>MAGAIKVGTWGGNGGSEWDMGPAYRIDSVKINAGDIIDAIEITFTRYGLTETQHYGGTGGEPHEIAFEDGEYIMSMEGHVVDYTGLTIIGKLTLTTNRRTFGPFGAYEGTPFSIPVAEGKIAGFFGRAGSFIDAIGVYLMPNLEHHHHHH[16x]

A BLAST protein sequence alignment search revealed a candidate lectin from Musa acuminata ssp. malaccensis, which we term Malayasian banana lectin (Malay BanLec). Like BanLec, Malay BanLec has a β-prism-I fold characteristic of the jacalin-related lectin family. To assess binding of WT versus F84T to HIV, we conducted surface plasmon resonance analysis to determine the binding times to, and binding avidities for, the gp140 trimer, which is made up of uncleaved ectodomains of the gp160 HIV envelope glycoprotein trimer. The results show that F84T and WT Malay BanLec, which like BanLec exist as dimers with two CBS per monomer (see Fig. 6 below and discussion thereof), bind with high avidity to the gp140 trimer. That is, we asked whether disruption of pi–pi stacking in a structurally related but distinct (only 63% identical at the amino acid level) jacalin-related lectin, Malaysian banana lectin (Malay BanLec), would reduce mitogenicity of the engineered lectin without abolishing antiviral activity.

We demonstrate that a single amino acid substitution, F84T, akin to the H84T mutation and predicted to remove the pi–pi stacking interaction, does indeed decrease mitogenicity while preserving antiviral activity. The F84T mutation in Malay BanLec disrupts pi–pi stacking without significant changes to the overall structure of the monomer or to the dimer. F84T and WT Malay BanLec have an almost identical structure, with an RMSD of 0.424 Å between all atoms. F84T Malay BanLec similarly loses pi–pi stacking (the “mitogenic wall”), but otherwise retains a structure that is almost identical to its parent lectin. We thus conclude that F84T is less mitogenic than is WT Malay BanLec because it likely does not crosslink surface molecules as well. F84T-treated cells also incorporated less BrdU than WT Malay BanLec-treated cells, indicating that F84T is less mitogenic than WT Malay BanLec. Taken together, these studies indicate that F84T induces less proliferation of PBLs, less expression of key cytokines/chemokines from PBMCs, and perhaps less activation of CD4 + PBMCs than WT Malay BanLec, indicating that F84T is less mitogenic than WT Malay BanLec. F84T robustly reduced luciferase activity, indicating that it retained the ability to inhibit HIV infection. As H84T is known to have broad-spectrum antiviral activity, we next sought to characterize whether F84T could inhibit additional viruses that are associated with human disease and are known to express mannose-containing N-glycans on their surfaces.> MSDPEQASPAATVQQTKAKYTKLPRPPIPEQTKRELWARAAGRCQFRGCNKLLYRDEVAKEAHNGATIAHIVAYSPDGPRGDTTRSEKLEKDISNLMLTCKTHGDHIDTLELVERYPEALLLEFKRDHEERVRNATAAVDSDKTTILIVQGAVSGKRVEVEPEQARKAIKPRWPANDGETLIDLNDLAIGEGRAAYWEVATEKIKAEAKQLLRRPAGQQPPQHLSIFALAPIPLLVLLGAEVNRVDVDLFQKHRGKSADTWCWDEGEPDADDDLKVFVPAELPGEIEDAAIIVSMTSIVDRKAVASAIGHPHHAFEIKARKPGPTFLKYRSQLTSFSNELYTILTTIRDDFRRVKRLHLILACPAPIAVEVGR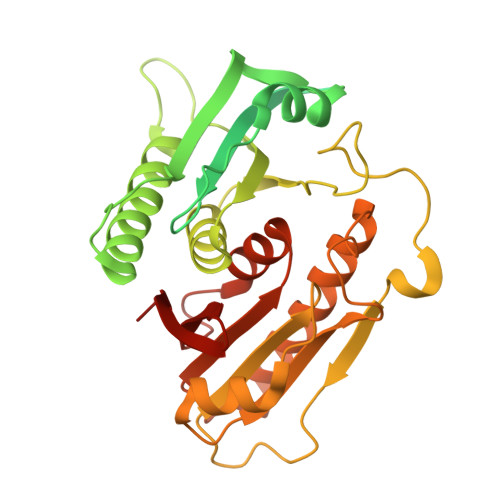SLIEKADPEAHVYEYLSPSYRRVLTINPKEGN> ATSDSNMLLNYVPVYVMLPLGVVNVDNVFEDPDGLKEQLLQ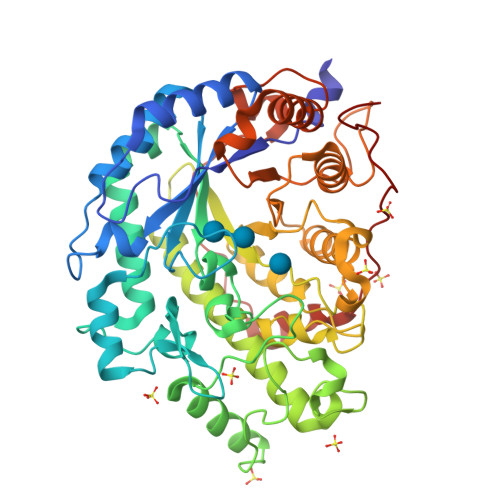LRAAGVDGVMVDVWWGIIELKGPKQYDWRAYRSLLQLVQECGLTLQAIMSFHQCGGNVGDIVNIPIPQWVLDIGESNHDIFYTNRSGTRNKEYLTVGVDNEPIFHGRTAIEIYSDYMKSFRENMSDFLESGLIIDIEVGLGPAGELRYPSYPQSQGWEFPGIGEFQCYDKYLKADFKAAVARAGHPEWELPDDAGKYNDVPESTGFFKSNGTYVTEKGKFFLTWYSNKLLNHGDQILDEANKAFLGCKVKLAIKVSGIHWWYKVENHAAELTAGYYNLNDRDGYRPIARMLSRHHAILNFACLEMRDSEQPSDAKSGPQELVQQVLSGGWREDIRVAGENALPRYDATAYNQIILNARPQGVNNNGPPKLSMFGVTYLRLSDDLLQKSNFNIFKKFVLKMHADQDYCANPQKYNHAITPLKPSAPKIPIEVLLEATKPTLPFPWLPETDMKVDG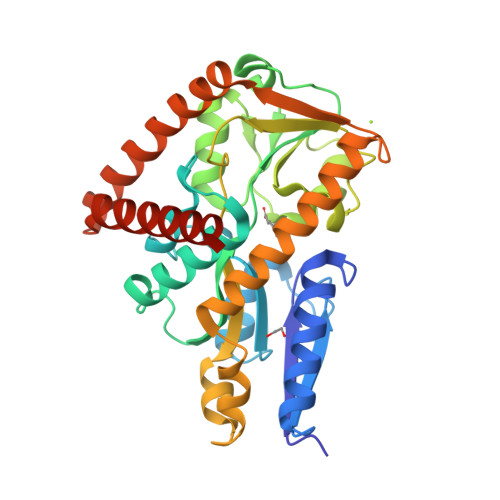>[2x]MQEAEYTLRLHHFFPASAPVHQEYFLPWKEAIEKESDGRLAVELYPSMQLGGTPPSLYDQAKDGQVDIIWTVLGYNSGRFPRAEVFDLPFLPTSGAATSQAAHEYAMTHMQDELEGVYPIAVHTHSPGALHTKETRIEALEDIEGLKMRGPSRLVNRYLAKLGAEPIGMPVAQALEALSRGVLDGTVIPFEAITAMGLADITTEHTIFSGDRALYTTMMIVAMDQDKYDALPEDLQPIIDAHAGGREAYRIGQIMDQADHRQILAIQSGEQPGTITRLGSEETARWQAVGQEVVDEWIAEAEEKGLDGQMLYDDATRLVERYTRAAALEHHHHHH> SLKVAPKVAVSAAAERVKLCPGAEDLEITKLPNGLIIASLENFSPASRIGVFIKAGSRYETTANLGTAHLLRLASPLTTKGASSFRITRGIEAVGGSLSVYSTREKMTYCVECLRDHVDTVMEYLLNVTTAPEFRPWEVTDLQPQLKVDKAVAFQSPQVGVLENLHAAAYKTALANPLYCPDYRIGKITSEQLHHFVQNNFTSARMALVGIGVKHSDLKQVAEQFLNIRSGAGTSSAKATYWGGEIREQNGHSLVHAAVVTEGAAVGSAEANAFSVLQHVLGAGPLIKRGSSVTSKLYQGVAKATTQPFDASAFNVNYSDSGLFGFYTISQAAHAGE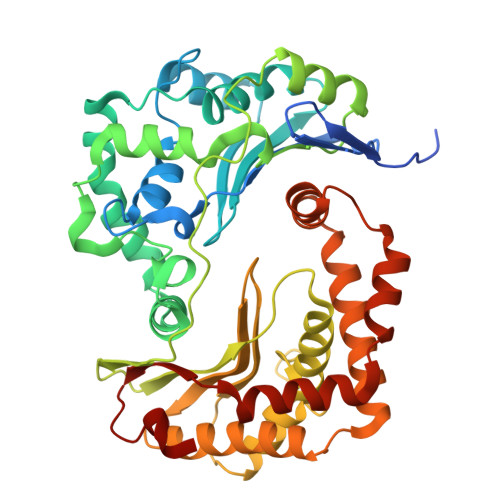VIRAAMNQLKAAAQGGVTEEDVTKAKNQLKATYLMSVETAQGLLNEIGSEALLSGTHTAPSVVAQKIDSVTSADVVNAAKKFVSGKKSMAASGDLGSTPFLDEL>[2x]SDGWTCAGSDFDGDQVRGQARHWVGQQKTKFSEFHTHNDVP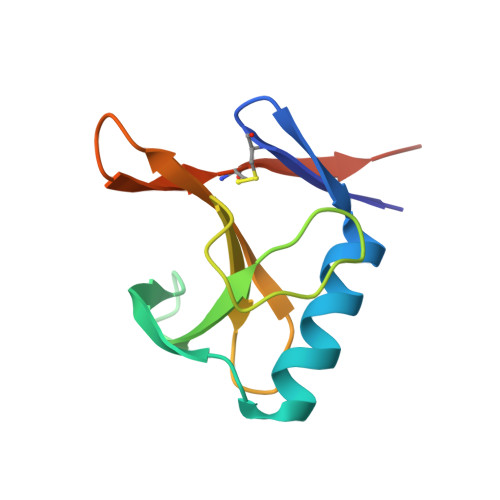LCYFELGEGNQLTQSYTGFRAYCDEPGDVYNLRYLDVSSRTWVLCTHYDNDFESDYR>[8x]GSMPRSSEGPLTGKVAFITGAARGQGRAHAVRLAADGADIIAVDLCDQIASVPYPLATPEELAATVKLVEDIGSRIVARQADVRDRESLSAALQAGLDELGRLDIVVANAGIAPMSAGDDGWHDVIDVNLTGVYHTIKVAIPTLVKQGTGGSIVLISSSAGLAGVGSADPGSVGYVAAKHGVVGLMRVYANLLAGQMIRVNSIHPSGVETPMINNEFTREWLAKMAAATDTPGAMGNAMPVEVLAPEDVANAVAWLVSDQARYITGVTLPVDAGFLNK

Here we present a series of TIGR03971 SDR crystal structures from several mycobacterial species which contain an insertion in the primary sequence at the NAD cofactor binding site. These crystal structures demonstrate that the inserted protein residues almost completely cover the NAD cofactor, only leaving part of the nicotinamide ring exposed to solvent. NMR experiments did not show exchange of the NAD cofactor, whereas binding was demonstrated for a number of small molecules which could be potential substrates, products, inhibitors, or artificial redox partners. Experimental results are consistent with the notion that the SDR family enzymes linked by comparative genomics studies to mycofactocin do indeed keep their NAD tightly bound beneath a protein structure that may interact with a specialized adaptor machinery for redox exchange.

With the exception of the M. thermoresistibile target which did not contain NAD, all other mycobacterial SDR target crystal structures contained NAD, which appears to have co-purified with the protein after expression in E. coli. For each of these crystal structures, the adenosine mononucleotide portion of the cofactor binding site is enveloped by the inserted residues and only a portion of the nicotinamide ring appears open to solvent (see representative examples in Fig. 2A and B). In addition to the insertion loop which covers the adenosine portion of the cofactor, a second loop which typically contains two α-helices covers much of nicotinamide mononucleotide portion of the cofactor. In contrast, this loop is ordered in each of the mycobacterial SDR crystal structures presented here. The combination of the insertion loop which covers the adenosine portion of the cofactor and the ordering of the second loop which covers the nicotinamide mononucleotide portion of the cofactor results in a significant decrease in the solvent accessible surface area of the cofactor in the mycobacterial SDRs, relative to other NAD- and NADP-dependent dehydrogenases. Only a small portion of the nicotinamide ring appears available to solvent in each of these cases, indicating that the NAD cofactor is tightly bound and potentially non-exchangeable. The structures presented here have a cofactor solvent accessible surface area of approximately 18 Å2, whereas other NAD- or NADP-bound dehydrogenases have a cofactor solvent accessible surface area of 82–89 Å2. Given the encapsulation of the NAD cofactor by the two loops in mycobacterial SDRs, a large conformational change would be required to release the NADH cofactor after a redox reaction had occurred. Alternatively, these structural elements may not allow for exchange of bound NAD/NADH with free NAD/NADH.>MILIADSGSTKTHWNVLDQGRVIGEIFTKGMNPFFQTPEEMGREIERTLLPQLNSNRFCEVHFFGAGCIPEKVPVVRNVLKGCLDVSSLIEVDTDMLAAAKASCGRSPGIVCIMGTGSNSCFYDGEKIAANVSPLGFILGDEGSGAVLGKLLIGDLLKNQMGEELKEKFLRQYELTPANIIERVYRQPFPNRFLAGISPFLAENIEHPAIHSLVLNAFKSFLTRNVMQFDYTRYKAHFIGSVAYYYKDILEEAAAATGIRTGTIVRNPMEGLRTYYSTVAKTV[2x]

Unlike other bacteria, the pathogenic Tannerella forsythia, a member of the red complex group of bacteria associated with the late stages of periodontitis, lacks biosynthetic pathways for MurNAc production and therefore obtains MurNAc from the environment. Sugar kinases play a crucial role in the MurNAc recycling process, activating the sugar molecules by phosphorylation. MurK and K1058 are two sugar kinases of the cell wall recycling system of T. forsythia, sharing a sequence identity of 44% and separated by a single PGN-scavenging operon within the genome. Structural and sequence data showed that MurK and K1058 both belong to the group of ribonuclease H-like kinases and are members of the ASKHA (acetate and sugar kinase/hsc70/actin) superfamily.

We successfully cocrystallised MurK with AMP-PCP (termed MurK/AMP-PCP) and established its structure at 2.12 Å resolution. Crystals of MurK/AMP-PCP were monoclinic and contain a biological dimer in the ASU. The AMP-PCP is clearly bound in both protomers of the ASU of the monoclinic crystals. AMP-PCP is bound at the N-terminal domain via a conserved DxGxT motif with interactions of the side chain of S9 upstream of the conserved T10 residue, both forming hydrogen bonds to the β-phosphate group. T116, also conserved in the homologs, is located on the opposite site of the phosphate entity and forms a hydrogen bond with the β-phosphate of AMP-PCP and the γ-phosphate to the backbone amino group of G117. The adenosine is bound mainly via van der Waals interactions contributed by nonpolar residues but forms hydrogen bonds via the carbonyl atom of A195 towards the hydroxy group at C2 atom of ribose and a water-mediated hydrogen bond via S198 to the adenosine ring system. In addition, the aromatic ring system is aligned coplanar to tightly pack against side chain Y244. Finally, S241, part of a conserved IGSV sequence (residues 238–241), stabilizes the α-phosphate by hydrogen bonding. Only minor rearrangements for ATP binding were observed, with an Cα-RMSD value of 0.78 Å, aligning all residues of the N-terminal domain of MurKapo and MurK in its AMP-PCP–bound state. This is in agreement with the observation that ATP is predominantly held in place by residues of the C-terminal domain.>GPNCAPGQKVKLFRASEPILSVLMWGVNHTINELSNVPVPVMLMPDDFKAYSKIKVDNHLFNKENLPSRFKFKEYCPMVFRNLRERFGIDDQDYQNSVTRSAPINSDSQGRCGTRFLTTYDRRFVIKTVSSEDVAEMHNILKKYHQFIVECHGNTLLPQFLGMYRLTVDGVETYMVVTRNVFSHRLTVHRKYDLKGSTVAREASDKEKA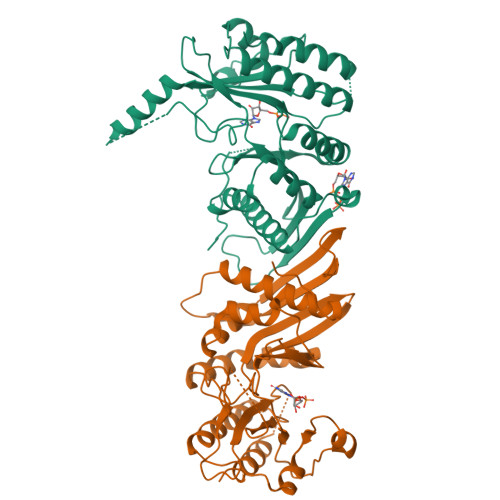KDLPTFKDNDFLNEGQKLHVGEESKKNFLEKLKRDVEFLAQLKIMDYSLLVGIHDVDRAEQEEMEVEERAEDEECENDGVGGNLLCSYGTPPDSPGNLLSFPRFFGPGEFDPSVDVYAMKSHESSPKKEVYFMAIIDILTPYDTKKKAAHAAKTVKHGAGAEISTVNPEQYSKRFNEFMSNILT[2x]N-{2-[TRANS-7-CHLORO-1-(2,2-DIMETHYL-PROPYL) -5-NAPHTHALEN-1-YL-2-OXO-1,2,3,5-TETRAHYDRO-BENZO[E] 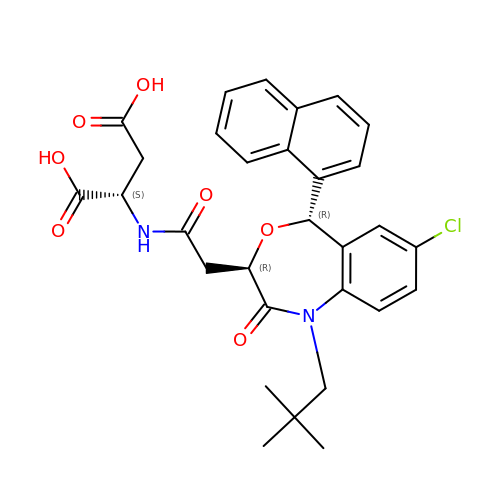[1,4]OXAZEPIN-3-YL]-ACETYL}-ASPARTIC ACID | C30 H31 Cl N2 O7 | GXDQAFKUUPODFF-CAKYRVLISA-N> HHHHHHALVCPAGWTLHGQRCFYSEATAMTWDLAEANCVNKGGHLASIHSLEEQLYIKDIVAGIVWIGGSACKVAGAWSW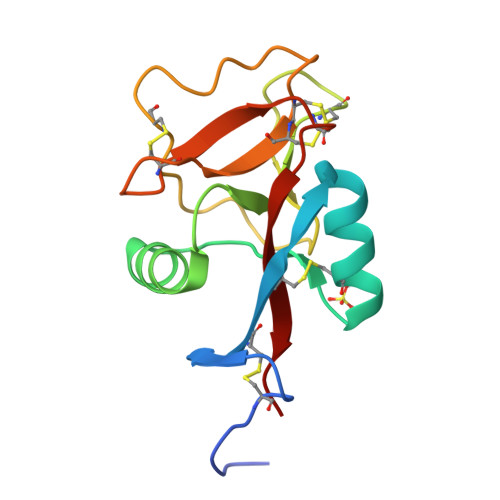TDGTPVDYRTWCPTKPNDILSDCCMQMTAAVDKCWDDLPCPASHASICAKAAI>[4x]RSRRVDVMDVMNRLILAMDLMNRDDALRVT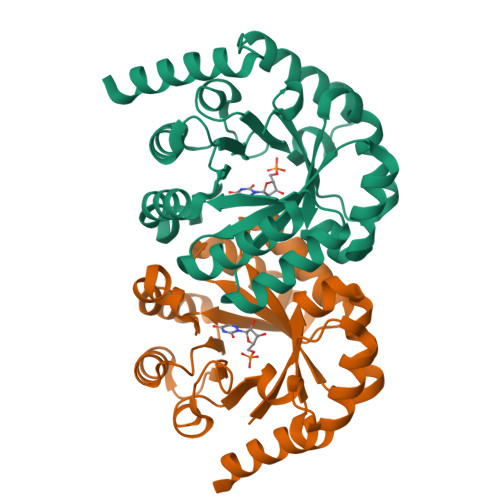GEVREYIDTVKIGYPLVLSEGMDIIAEFRKRFGCRIIADFKVADIPETNEKICRATFKAGADAIIVHGFPGADSVRACLNVAEEMGREVFLLTEMSHPGAEMFIQGAADEIARMGVDLGVKNYVGPSTRPERLSRLREIIGQDSFLISPGVGAQGGDPGETLRFADAIIVGRSIYLADNPAAAAAGIIESIKDLLIPEDPAANKARKEAELAAATA> SVRPWEFRKVIQAEYRERLPRNYELKHWKKPSKIMIGSILRLLETNTVSALDSVFEKYEKEMNQMTHGDNNEVKRIYSKKERLLEIILTKIKKKLRQAKFPSRISERDLDIEYIYSKRQFIQNRYSQELQNNERLEAILSREQNLLEETRKL;> LSSSITSVTTIDVLSSLFINLFENDLIPQALKDFNKSDDDQFRKLLYKLDLRLFQTISDQMTRDLKDILDINVSNNELCYQLKQVLARKEDLNQQIISVRNEIQELK;> QSINDRALSLLQRTRATK

Kinetochores assemble at centromeres by interacting with a variant histone H3 known as centromere protein A (CENP‐A) in vertebrates and as Cse4 in Saccharomyces cerevisiae and other point‐centromere yeast. More recent biochemical reconstitution experiments showed that the Okp1‐Ame1 heterodimer, which is a Ctf19c sub‐module that binds the Ctf19 protein, is the direct binding partner of Cse4END (Anedchenko et al, 2019; Fischbock‐Halwachs et al, 2019; Hinshaw & Harrison, 2019). Okp1 and Ame1 are the only Ctf19c components fully required for mitosis (Ortiz et al, 1999; Pot et al, 2005). They associate as an elongated heterodimer with a globular “head” and an extended alpha‐helical coiled‐coil “shaft.

We determined a 1.8 Å resolution crystal structure of a truncated Okp1‐Ame1 bound with a Cse4END peptide to specify in detail the amino acid residues involved, and we have shown by binding experiments and yeast genetics that the interaction is functionally relevant in cells. We determined the crystal structure of the Cse4END peptide bound to a minimal Okp1‐Ame1 heterodimer. Crystals containing all three proteins, including the full Cse4END sequence, grew in space group P 42212 (Fig EV1A and B) and yielded diffraction data to a minimum Bragg spacing of 1.8 Å. The ordered Cse4 residues in the crystal structure are mostly α‐helical (residues 34–46). The three‐way interface between Cse4, Okp1, and Ame1 has a hydrophobic core surrounded by polar interactions. Hydrophobic contacts between Cse4 and Okp1 include Cse4‐L42 and Okp1‐I234. Likewise, Cse4‐L41 and ‐I34 contact Ame1 I195. Peripheral charged contacts include an electrostatic interaction between Cse4‐R46 and Okp1‐E235. Cse4‐R37 makes complementary charge contacts with Ame1‐D191 and ‐D194. In the current structure, the Okp1‐Ame1 head tilts away from the shaft.>MRFILTGVPGAGKTTVCNKLAEKMSNLSVVNYGDVIFEEAKKLYPSIIQVREDTRKLPRADYRNIQIEAAKKISLITDNLIVDTHMSLKTPYGFYPGLIPETINIIQPDGIILLEFNPRDVIARREKDRLAGKRVTRDMESETDILLHQQVNRMFAVSYSAINQCYVKIIDLTWPQEYEFQHTEYAVNKIIEMLNFKI[6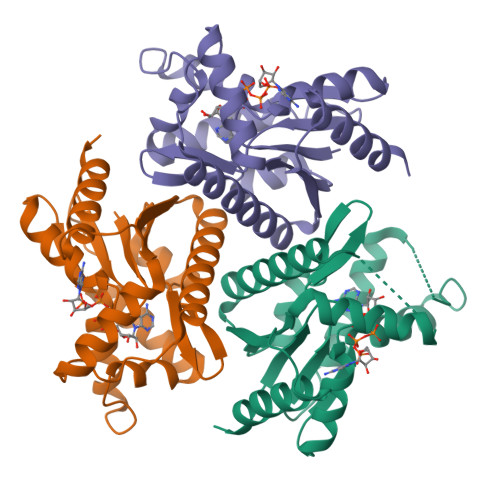x]>GSHMWVQRVKEKEAELKEAEKELHEKFDRLKKLHQDEKKKLEDKKKSLDDEVN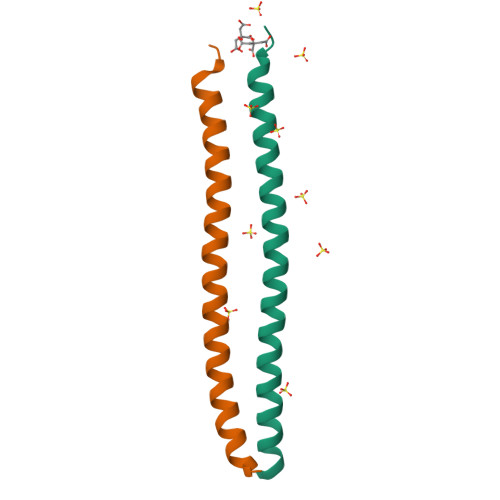AFKQR[2x]2-(3-fluoranylphenoxy)-~{N}-(4-pyridin-2-yl-1,3-thiazol-2-yl)ethanamide | C16 H12 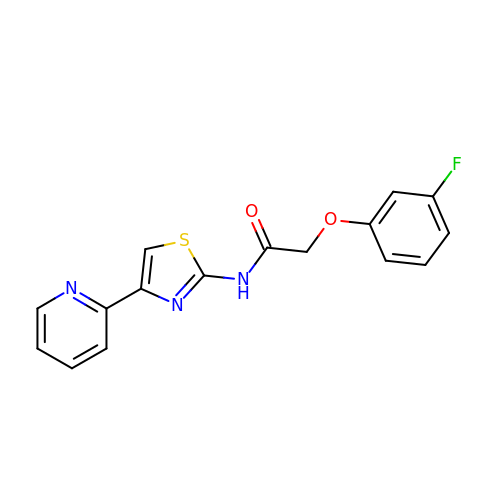F N3 O2 S | NMSQSTANKRXRFA-UHFFFAOYSA-N>MAGTDKRKQSLYFPEEMLKEIQEEATRQDRSLSWVVQQAWKIARERIKSFPAVNDVTGDERQDPREE[3x]

We show that CdbA is a tetrameric ribbon-helix-helix DNA binding protein and changes conformation upon c-di-GMP binding. Consistently, c-di-GMP and DNA binding are mutually exclusive. In vivo CdbA is essential, while CdbB is not, and depletion of CdbA causes defects in chromosome organization and segregation resulting in defects in cell division. CdbA is abundant and binds globally to the M. xanthus chromosome. These observations are in agreement with a model whereby CdbA is a ligand-regulated nucleoid-associated protein (NAP) important for chromosome organization and segregation and in which CdbA activity is modulated by c-di-GMP.

We obtained two crystal forms of full-length CdbA-His6. Successful model building of the first form allowed us to solve the second form via molecular replacement. This form has three copies of the protein in the asymmetric unit, one of which forms a tetramer via crystallographic symmetry (four copies of same chain) and two of which form a dimer within the asymmetric unit, which then tetramerizes over the final crystallographic axis. The tetramer centers on residue F50 of the two innermost chains, and the C-terminal tails can be traced five residues further than in form one, and with the C-terminal tail of the innermost chains in a dimer contacting an opposing dimer. Protein–protein contacts mediated by the tail region include a hydrophobic component from F50 and V53 in one chain projecting towards a pocket in the opposing dimer formed by W34/I42/I47, a second hydrophobic interaction between V56 and P14/M17, and a more polar interface between the free carbonyl groups of A52/V53/D55 and the side chains of Q38 and K41. The arrangement of the two dimers in the tetramer places their β-sheets ~35 Å apart (measured between Cα atoms of equivalent Y12 residues). Using the RHH protein Arc, which binds DNA as a tetramer and with the two β-sheets separated by 26Å40,41, as a template, we created a model of how CdbA could bind DNA. Because the β-sheets are ~35 Å apart in CdbA, this model suggests that CdbA bends DNA upon binding. The tetramer interface displays different hydrophobic packing between the two crystal forms we observed here, suggesting that it may have inherent plasticity that allows it to undergo this change.In the present study, we perform a detailed biochemical characterization of the BAI1/ELMO2 interaction, and find that an evolutionarily conserved fragment located in the intracellular region of BAI1 specifically binds to the RBD-ARR-ELMO (RAE) tandem of ELMO2. To elucidate the assembly of BAI1/ELMO2 complex, we solve the crystal structures of the RAE tandem of ELMO2 and its complex with BAI1 at 2.5-Å and 1.7-Å resolutions, respectively. The RBD, ARR and ELMO domains of ELMO2 bind tightly and form a structural and functional supramodule, creating a highly conserved elongated concave groove capable of specifically binding to the BAI1 fragment. Each member consists of the Ras-binding domain (RBD), the armadillo repeats domain (ARR), the engulfment and motility (ELMO) domain, the pleckstrin homology (PH) domain and the C-terminal proline rich region (PRR).

Diffraction-quality crystals of ELMO-RAE belong to the C2221 space group. In the structure, the ELMO2-RAE forms an elongated superhelical architecture that consists of three domains: the N-terminal RBD domain (aa 1-80), the ARR domain (aa 81-301), and the ELMO domain (aa 306-513). The RBD domain adopts a typical ubiquitin-like superfold, which closely resembles the RBD of FHOD1, consistent with the previous bioinformatic analyses. The ARR domain contains five armadillo repeats (ARMs), though the ARM-1 is not complete. The ELMO domain has an all α-helical topology, composed of 11 α-helices. A Dali26 search suggests that the ELMO domain represent a novel fold with a global architecture. Notably, a 16-residue flexible loop (421LQVGELPNEGRNDYHP436) between α6 and α7 of the ELMO domain interacts tightly with the ARR domain (see below for the detail). In the RBD-ARR binding interface, Y60RBD inserted into the hydrophobic pocket formed by Pro81, Ala84, Leu88, Leu110, and Phe116 from ARR domain, which is similar to RBD-ARR interface occurred in FHOD1. The ARR-ELMO binding interface could be separated into two parts: (1) a 16-residue flexible loop between α6 and α7 of ELMO domain forms extensive hydrogen bonds with the residues from α14 of ARR domain, such as H284ARR-R431ELMO and N295ARR-E425ELMO interactions. (2) the distal side of ARR domain binds tightly to ELMO domain via extensive hydrophobic interactions. The second interface is further reinforced by additional polar interactions like R264ARR-D442 ELMO and R300ARR-D375ELMO pairs. It is worth noting that most of the residues involved in the binding interfaces are conserved among the ELMO family proteins, suggesting that the supramodular folding of RAE tandem is a common feature for all ELMOs.

> GPGSMPPPSDIVKVAIEWPGANAQLLEIDQKRPLASIIKEVCDGWSLPNPEYYTLRYADGPQLYITEQTRSDIKNGTILQLAISPSRAARQLMERTQSSNMETRLDAMKELAKLSADVTFATEFINMDGIIVLTRLVESGTKLLSHYSEMLAFTLTAFLELMDHGIVSWDMVSITFIKQIAGYVSQPMVDVSILQRSLAILESMVLNSQSLYQKIAEEITVGQLISHLQVSNQEIQTYAIALINALFLKAPEDKRQDMANAFAQKHLRSIILNHVIRGNRPIKTEMAHQLYVLQVLTFNLLEERMMTKMDPNDQAQRDIIFELRRIAFDAESDPSNAPGSGTEKRKAMYTKDYKMLGFTNHINPAMDFTQTPPGMLALDNMLYLAKVHQDTYIRIVLENSSREDKHECPFGRSAIELTKMLCEILQVGELPNEGRNDYHPMFFTHDRAFEELFGICIQLLNKTWKEMRATAEDFNKVMQVVREQITRALPSKPNSLDQFKSKLRSLSYSEILRLRQSERMSQDD> MAMKAYSMLNVTATLDGRRVIGLMDGDDAITTSPGVDVGTMLVGADGSWLFSQTADKSATVVIKLKPNSPTHRQLTEKWMAQRAGRLVGFPFD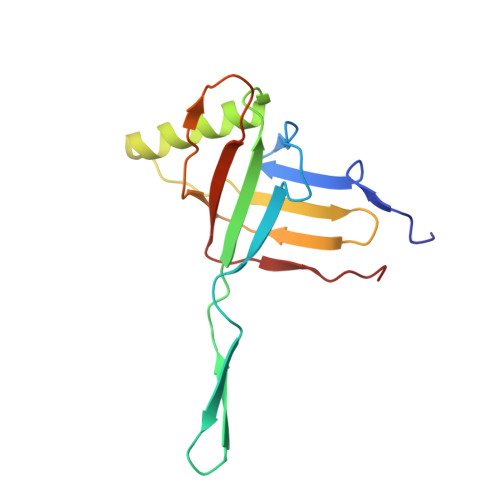FIDSASNEGGTGAEFFIQKAPDDSKGNNAVVREWTIVTGEWTPTIPTLL>[4x]MTTTTTKKPHVLVIPFPQSGHMVPHLDLTHQILLRGATVTVLVTPKNSSYLDALRSLHSP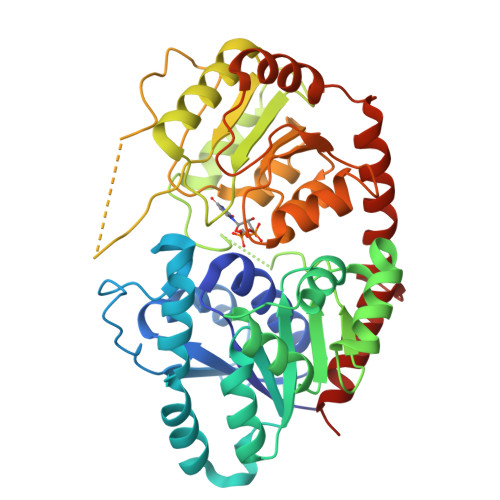EHFKTLILPFPSHPCIPSGVESLQQLPLEAIVHMFDALSRLHDPLVDFLSRQPPSDLPDAILGSSFLSPWINKVADAFSIKSISFLPINAHSISVMWAQEDRSFFNDLETATTESYGLVINSFYDLEPEFVETVKTRFLNHHRIWTVGPLLPFKAGVDRGGQSSIPPAKVSAWLDSCPEDNSVVYVGFGSQIRLTAEQTAALAAALEKSSVRFIWAVRDAAKKVNSSDNSVEEDVIPAGFEERVKEKGLVIRGWAPQTMILEHRAVGSYLTHLGWGSVLEGMVGGVMLLAWPMQADHFFNTTLIVDKLRAAVRVGENRDSVPDSDKLARILAESAREDLPERVTLMKLREKAMEAIKEGGSSYKNLDELVAEMCL>MASLNTPAPLPTSCNPSDMSHGYVTVKPRVRLHFVELGSGPAVCLCHGFPESWYSWRYQIPALAQAGYRVLAMDMKGYGESSAPPEIEEYCMEVLCKEMVTFLDKLGLSQAVFIGHDWGGMLVWYMALFYPERVRAVASLNTPFIPANPNMSPL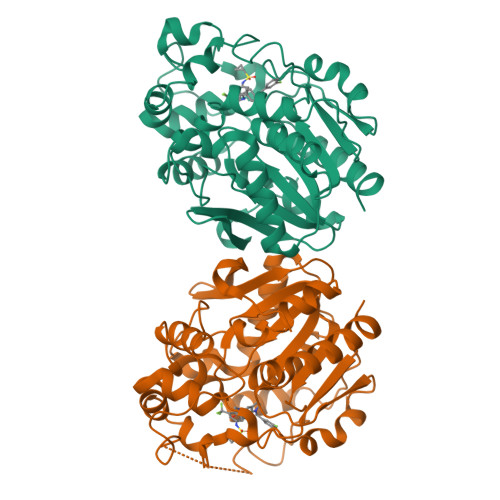ESIKANPVFDYQLYFQEPGVAEAELEQNLSRTFKSLFRASDESVLSMHKVCEAGGLFVNSPEEPSLSRMVTEEEIQFYVQQFKKSGFRGPLNWYRNMERNWKWACKSLGRKILIPALMVTAEKDFVLVPQMSQHMEDWIPHLKRGHIEDCGHWTQMDKPTEVNQILIKWLDSDARNPPVVSKMLLEHHHHHH[2x]> MAIGLKAYPELCHGCGNCVIACPVNALRSPEVAGGKGPTDDVEIIMI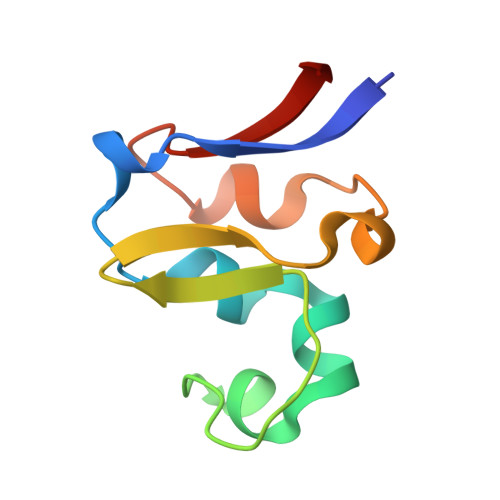VEDGVVNIKNPDLCGKCGTCVESCPVDAIRLEELE> MSSNTSSVMSSPRVEKRSFSSTLKSFFTNPNKKRPSSKKVFSSNLSYANHLEESDVEDTLHVNKRKRVSGTSQHSDSLTQNNNNAPIIIYGTENTERPPLLPILPIQRLRLLREKQRVRNMRELGLIQSTEFPSITSSVILGSQSKSDEGGSYLCTSSTPSPIKNGSCTRQLAGKSGEDTNVGLPILKSLKNRSNRKRFHSQSKGTVWSANFEYDLSEYDAIQKKDNKDKEGNAGGDQKTSENRNNIKSSISNGNLATGPNLTSEIEDLRADINSNRLSNPQKNLLLKGPASTVAKTAPIQESFVPNSERSGTPTLKKNIEPKKDKESIVLPTVGFDFIKDNETPSKKTSPKATSSAGAVFKSSVEMGKTDKSTKTAEAPTLSFNFSQKANKTKAVDNTVPSTTLFNFGGKSDTVTSASQPFKFGKTSEKSENHTESDAPPKSTAPIFSFGKQEENGDEG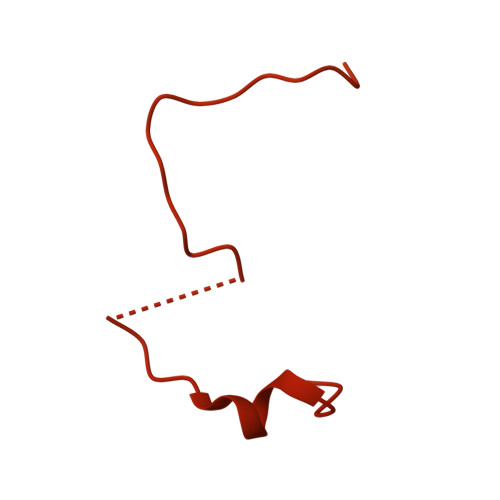DDENEPKRKRRLPVSEDTNTKPLFDFGKTGDQKETKKGESEKDASGKPSFVFGASDKQAEGTPLFTFGKKADVTSNIDSSAQFTFGKAATAKETHTKPSETPATIVKKPTFTFGQSTSENKISEGSAKPTFSFSKSEEERKSSPISNEAAKPSFSFPGKPVDVQAPTDDKTLKPTFSFTEPAQKDSSVVSEPKKPSFTFASSKTSQPKPLFSFGKSDAAKEPPGSNTSFSFTKPPANETDKRPTPPSFTFGGSTTNNTTTTSTKPSFSFGAPESMKSTASTAAANTEKLSNGFSFTKFNHNKEKSNSPTSFFDGSASSTPIPVLGKPTDATGNTTSKSAFSFGTANTNGTNASANSTSFSFNAPATGNGTTTTSNTSGTNIAGTFNVGKPDQSIASGNTNGAGSAFGFSSSGTAATGAASNQSSFNFGNNGAGGLNPFTSATSSTNANAGLFNKPPSTNAQNVNVPSAFNFTGNNSTPGGGSVFNMNGNTNANTVFAGSNNQPHQSQTPSFNTNSSFTPSTVPNINFSGLNGGITNTATNALRPSDIFGANAASGSNSNVTNPSSIFGGAGGVPTTSFGQPQSAPNQMGMGTNNGMSMGGGVMANRKIARMRHSKR>[4x]MSSKPTDRGQQYKDGKFTQPFSLVNQPD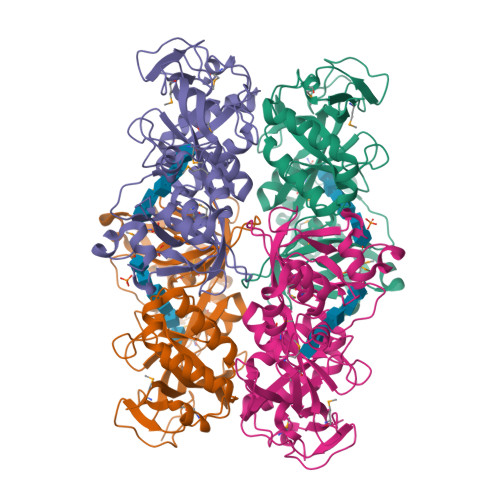AVGAPINAGDFAEQINHIRNSSPRLYGNQSNVYNAVQEWLRAGGDTRNMRQFGIDAWQMEGADNYGNVQFTGYYTPVIQARHTRQGEFQYPIYRMPPKRGRLSSRAEIYAGALSDKYILAYSNSLMDNFIMDVQGSGYIDFGDGSPLNFFSYAGKNGHAYRSIGKVLIDRGEVKKEDMSMQAIRHWGETHSEAEVRELLEQNPSFVFFKPQSFAPVKGASAVPLVGRASVASDRSIIPPGTTLIAEVPLLDNNGKFNGQYELRLMVALDVGGAIKGQHFAIYQGIGPEAGHRAGWYNHYGRVWVLKTAPGAGNVFSG> MASWSHPQFEKIEGRH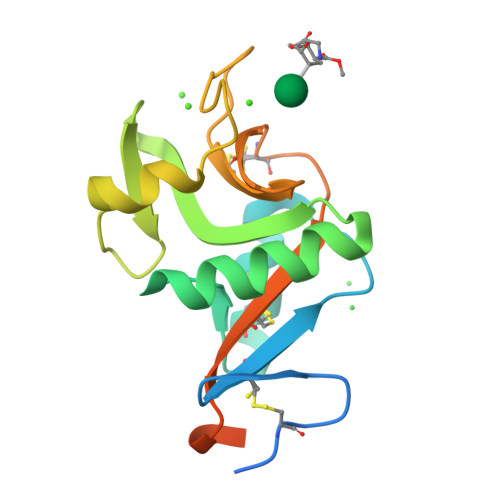PCPWEWTFFQGNCYFMSNSQRNWHDSITACKEVGAQLVVIKSAEEQNFLQLQSSRSNRFTWMGLSDLNQEGTWQWVDGSPLLPSFKQYWNRGEPNNVGEEDCAEFSGNGWNDDKCNLAKFWICKKSAASCSRDEEQFLSPAPATPNPPPA> GSHMNLKEQLCFSLYNAQRQVNRYYSNKVFKKYNLTYPQFLVLTILWDESPVNVK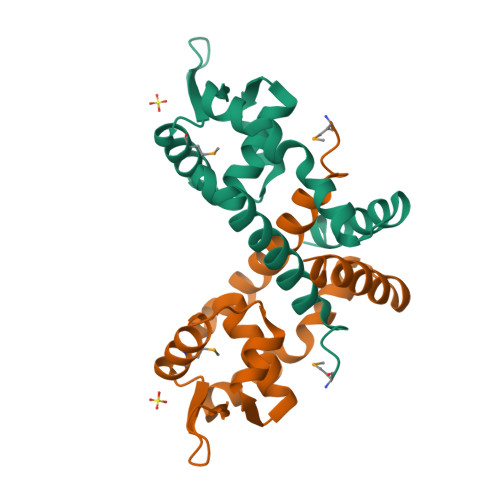KVVTELALDTGTVSPLLKRMEQVDLIKRERSEVDQREVFIHLTDKSETIRPELSNASDKVASASSLSQDEVKELNRLLGKVIHAFDE HPV E7 is composed of three conserved regions (CRs): CR1 at the N-terminal end; CR2, which follows CR1 and contains the LxCxE motif; and CR3 comprising the C-terminal half of the protein. Unlike CR1 and CR2, which are known to be unstructured, CR3 forms a homodimeric domain structure whose monomer is composed of two α-helices and two β-strands, in which a zinc ion is coordinated. PTPN14 is a cytosolic PTP protein and constitutes a tumor-suppressive p53–PTPN14–yes-associated protein (YAP) axis that controls the Hippo signaling pathway.

In this study, we confirmed the direct and potent interaction between the two domains and determined the crystal structure of the PTP domain of human PTPN14 in a complex with the C-terminal domain of HPV18 E7. The resulting dissociation constant (KD) of the interaction was determined to be 18.2 nM, demonstrating that they interact with each other with remarkably high binding affinity. Next, we attempted the crystallization of the PTPN14 PTP domain in a complex with the HPV18 E7 C-terminal domain, which consequently led to the determination of the complex structure to a resolution of 1.8 Å. The PTP domain of PTPN14 contains a central twisted β-sheet composed of eight β-strands, which is surrounded by seven α-helices. The HPV18 E7 C-terminal domain is composed of two α-helices and two antiparallel β-strands, in which a zinc ion is captured by four cysteine residues provided from two CXXC motifs (C65CKC68 and C98PWC101). The intermolecular interactions between the two proteins are mainly mediated by α1 and β1 from the HPV18 E7 C-terminal domain and β5, β6, β7, and α4 from the PTPN14 PTP domain. In detail, intermolecular hydrophobic interactions involve Phe90 and Leu91 from α1 and Met61 and Leu62 from β1 of HPV18 E7 and Lys1043 and Phe1044 from β5, Gly1055 from β6, Trp1070 from β7, and Leu1026 from the β3–β4 loop of PTPN14. Additionally, Arg84 from α1 of HPV18 E7 constitutes an electrostatic interaction with Glu1095 from α4 of PTPN14. The interaction of HPV18 E7 does not induce a dramatic conformational change of the PTPN14 PTP domain, as its structures in the apo form and in the HPV18 E7–bound form were well matched when superimposed with a root-mean-square deviation (RMSD) value of 0.93 Å over 276 aligned residues. Moreover, the conformation of main and side chains of the phosphate-binding loop containing the catalytic cysteine residue (Cys1121 of PTPN14) and the tryptophan-proline-aspartate (WPD) loop containing the general/acid base aspartate residue (Asp1079 of PTPN14), both of which are critical for the catalytic activity of the PTP protein, are not notably altered upon binding to HPV18 E7.

> MVDATRVPMDERFRTLKKKLEEGMVFTEYEQIPKKKANGIFSTAALPENAERSRIREVVPYEENRVELIPTKENNTGYINASHIKVVVGGAEWHYIATQGPLPHTCHDFWQMVWEQGVNVIAMVTAEEEGGRTKSHRYWPKLGSKHSSATYGKFKVTTKFRTDSVCYATTGLKVKHLLSGQERTVWHLQYTDWPDHGCPEDVQGFLSYLEEIQSVRRHTNSMLEGTKNRHPPIVVHCSAGVGRTGVLILSELMIYCLEHNEKVEVPMMLRLLREQRMFMIQTIAQYKFVYQVLIQFLQNSRLI;> GHMAEPQRHTMLCMCCKCEARIELVVESSADDLRAFQQLFLNTLSFVCPWCASQQ(1~{R},3~{S},5~{Z})-4-methylidene-5-[(~{E})-3-[3-(6-methyl-6-oxidanyl-heptyl)phenyl]hept-2-enylidene]cyclohexane-1,3-diol | C28 H42 O3 | 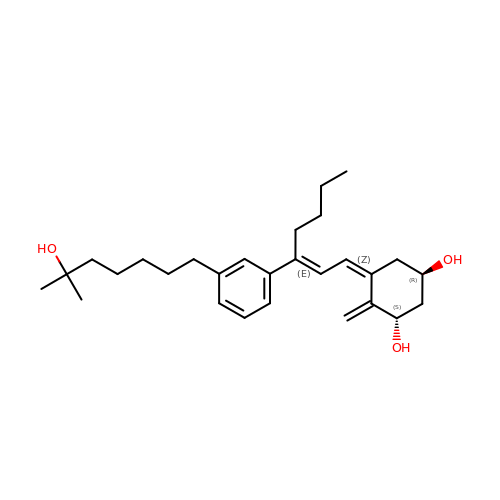UWAWDTCFOCGFNY-NTWKYLMFSA-N Natural resistance-associated macrophage proteins (Nramps) are APC-superfamily transition metal transporters that enable uptake of rare micronutrients such as Mn2+ in plants and bacteria and Fe2+ in animals. Nramps bind and/or transport biologically-essential divalent metals such as Mn2+, Fe2+, Co2+, Ni2+, Cu2+, Zn2+—and toxic metals like Cd2+, Pb2+, and Hg2+—but not the abundant alkaline earth metals Mg2+ and Ca2+. Metal uptake by Nramps is typically stimulated by acidic pH and accompanied by proton influx. Nramps have 11 or 12 TMs, the first ten forming a LeuT fold, as seen in structures of three bacterial Nramp homologs, including our model system Deinococcus radiodurans (Dra)Nramp.

We chose to pursue G223W—on TM6a one helical turn above the unwound metal-binding region—which like G45R eliminated Co2+ and Fe2+ metal transport. Importantly, a tryptophan modeled in the inward-open DraNramp Patch mutant structure at position 223 clashes with the top of TM10. In contrast, G223W significantly increased A61C accessibility while fully protecting A53C, consistent with an outward-locked state. We also determined a G223W apo structure, which lacks electron density attributable to metal substrate in the binding site but is otherwise similar to the metal-bound state (Cα RMSD = 1.08 Å); hence we used the metal-bound structure for all further analyses. The G223W ΔN34 apo dataset compiled from many small crystals is 96% complete to 4.5 Å, 92% complete to 3.4 Å, 77% complete to 3.0 Å, 66% complete to 2.85 Å, and 52% complete to 2.7 Å. Compared to the inward-open and inward-occluded structures, in the outward-open state TM1b, TM6a, and the top of TM10 are splayed open, and loop 1–2 is displaced by ~4 Å, to form a wide aqueous pathway to the metal-binding site. On the cytoplasmic side, TM4 and TM5 move significantly (by ~8 Å) straddling TM8 and approaching TM1a, while TM1a also approaches TM8 to fully shut the interior aqueous vestibule. Surprisingly, in the presence of a favorable negative membrane potential established using K+ gradients and the K+-ionophore valinomycin, G223W enabled larger basal H+ influx than WT, while G45R had no H+ flux. As the transporter reaches the outward-open state seen in EcoNramp and our apo G223W structure, a protonation event at D56 may prime the binding site to receive another incoming metal ion.

> MHHHHHHHHMRGVRRILPFLGPAVIASIAYMDPGNFATNIEGGARYGYSLLWVILAANLMAMVIQNLSANLGIASGRNLPELIRERWPRPLVWFYWIQAELVAMATDLAEFLGAALAIQLLTGLPMFWGAVVTGVVTFWLLNLQKRGTRPLELAVGAFVLMIGVAYLVQVVLARPDLAAVGAGFVPRLQGPGSAYLAVWIIGATVMPHVIYLHSALTQGRIQTDTTEEKRRLVRLNRVDVIAAMGLAGLINMSMLAVAAATFHGKNVENAGDLTTAYQTLTPLLGPAASVLFAVALLASGLSSSAVGTMAGDVIMQGFMGFHIPLWLRRLITMLPAFIVILLGMDPSSVLILSQVILCFGVPFALVPLLLFTARRDVMGALVTRRSFTVIGWVIAVIIIALNGYLLWELLGG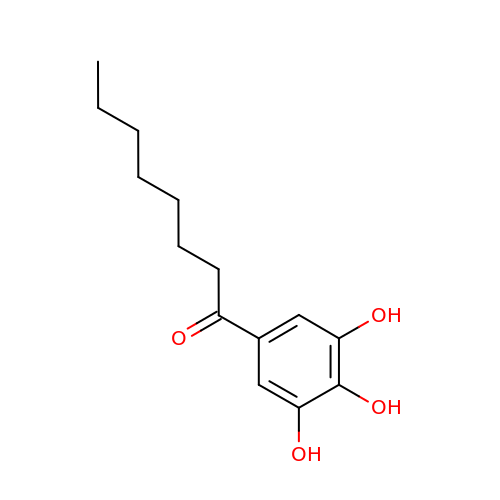1-(3,4,5-trihydroxyphenyl)octan-1-one | C14 H20 O4 | XPNDSNQZWXZZAW-UHFFFAOYSA-N> KLHYTTMIMTQFPDISIQSVESLGEGFRNYAILVNGDWVFRFPKSQQGADELNKEIQLLPLLVGCVKVNIPQYVYIGKRSDGNPFVGYRKVQGQILGEDGMAVLPDDAKDRLALQLAEFMNELSAFPVETAISAGVPVTNLKNKILLLSEAVEDQVFPLLDESLRDYLTLRFQSYMTHPVYTRYTPRLIH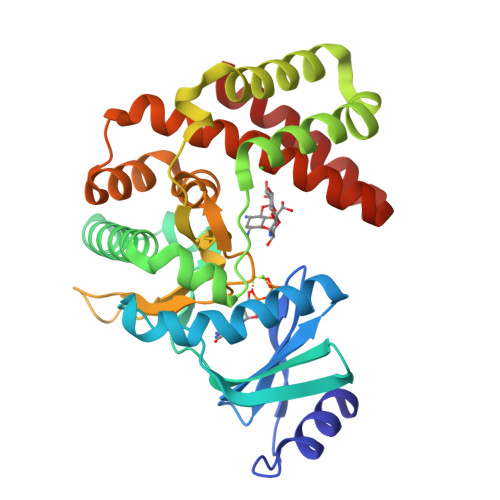GDLSPDHFLTNLNSRQTPLTGIIDFGDAAISDPDYDYVYLLEDCGELFTRQVMAYRGEVDLDTLIRKVSLFVTFDQVSYLLEGLRARDQDWISEGIELLEEDKANNF> MPKLVTWMNNQRVGELTKLANGAHTFKYAPEWLASRYARPLS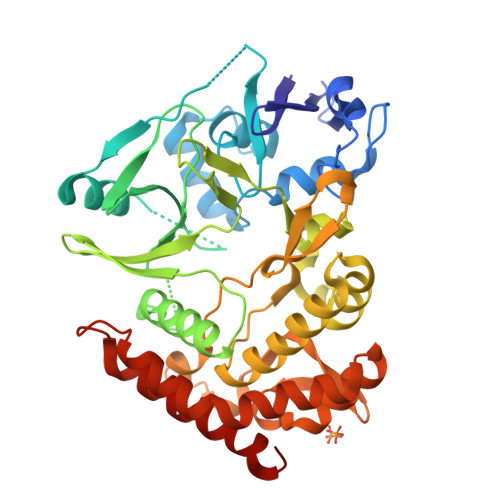LSLPLQRGNITSDAVFNFFDNLLPDSPIVRDRIVKRYHAKSRQPFDLLSEIGRDSVGAVTLIPEDETVTHPIMAWEKLTEARLEEVLTAYKADIPLGMIREENDFRIAVAGAQEKTALLRIGNDWCIPKGITPTTHIIKLPIGEIRQPNATLDLSQSVDNEYYCLLLAKELGLNVPDAEIIKAGNVRALAVERFDRRWNARRTVLLRLPQEDMCQTFGLPSSVKYESDGGPGIARIMAFLMGSSEALKDRYDFMKFQVFQWLIGATQGHAKNFSVFIQAGGSYRLTPFYDIISAFPVLGGTGIHISDLKLAMGLNASKGKKTAIDKIYPRHFLATAKVLRFPEVQMHEILSDFARMIPAALDNVKTSLPTDFPENVVTAVESNVLRLHGRLSREYGSK> 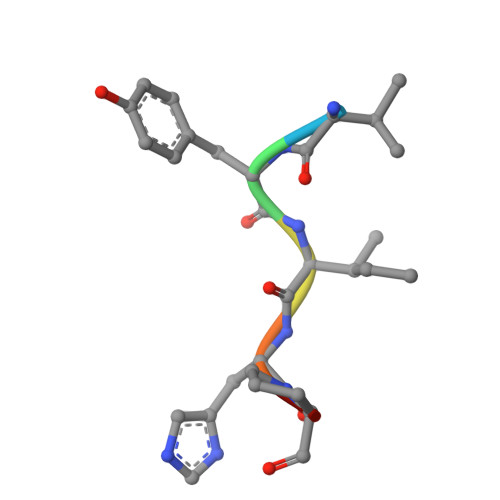VYIHPF>MSKLVLTGERHYTRNDDIRQSILALGEPGTFMTQDVNIIQTQIEQRLPWIKQVSVRKQWPDELKIHLVEYVPIARWNDQHMVDAEGNTFSVPPERTSKQVLPMLYGPEGSANEVLQGYREMGQMLAKDRFTLKEAAMTARRSWQLTLNNDIKLNLGRGDT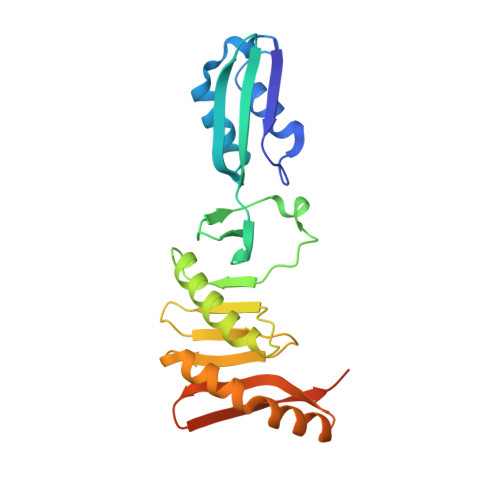MKRLARFVELYPVLQQQAQTDGKRISYVDLRYDSGAAVGWAPLPPEESTQQQNQAQAEQQ[2x]BUTENOIC ACID | C4 H6 O2 | 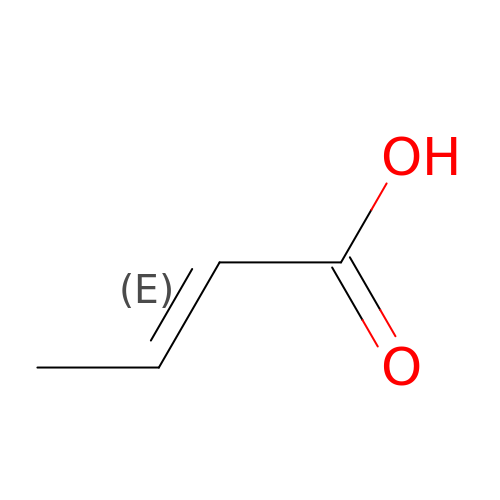LDHQCZJRKDOVOX-NSCUHMNNSA-N> MKKESINTSGPDNTKSSISDEIEISNEISWTALSGVISAANNADGRLEVFGVGTNNAVWHNWQTVPNTGSSWSGWHSLNEGATSKPAVHINSDGRLEVFVRGTDNALWHNWQTVPGAGWSGWQSLGGQITSNPVVYINSDGRLEVFARGADNALWHIWQTAPHAGPWSNWQSLNGVLTSDPTVYVNASGRPEVFARSNDYSLWYIKQTASHTYPWTNWQSLSGVITSNPVVISNSDGRLEVFARGSDNALWHIWQVAPNAGWTNWRSLSGIITSDPAVHINADGRLEVFARGPDNALWHIWQTATSDAWSEWTSLSGVITSAPTVAKNSDGWLEVFARGANNALCHIQQTTSSWSTWTSLGGNLIDASAIK

In this article, we studied five members of the PLL lectin family from P. laumondii subsp. laumondii TT01 (PLL, PLL2, PLL3, PLL4, PLL5, collectively referred to as PLLs). All studied lectins belong to the seven-bladed β-propeller structural family. Each blade makes a W-motif composed of four antiparallel beta-strands (β1-β4) connected by β-turns and loops. The saccharide binding sites are located between the adjacent blades and are uniquely organized in two separate circles around the monomer.

The lowest avidity effect can be seen for PLL3, the only monomeric protein in this family. Residues involved in ligand binding are highly conserved throughout the PLL family. The orientation of the ligand in the H-type binding site is consistent across all PLLs (Fig. 8F - an example of PLL3-4H site). C6 of αMeFuc points inside the binding pocket, where it is stabilized via hydrophobic interaction. Two highly conserved tryptophans (e.g. W265 and W251 in PLL3-4H site) are essential in stabilizing the ligand via CH-π stacking interaction with C6, C5, and C4. Additional ligand stabilization is formed by a hydrogen bond between O3 and the side chain of the polar amino acid (Ser/Thr; e.g. S246 in PLL3-4H site) if presented in the β-turn T2. The methyl group on C1 of methyl-α-l-fucoside ligand is oriented towards the solvent, providing sufficient space to accommodate potential binding of methyl-β-l-fucoside in the H sites of PLLs. The ligand in the P-type binding site has a distinct orientation, where C6 is pointing outside the binding pocket (Fig. 8E - an example f PLL3-2P site). Delocalized electrons of the tryptophan (e.g. W111 in PLL3-2P site) are involved in the stabilization of C3, C4 and C5 via CH-π stacking interaction. In human blood activated by zymosan A, PLL2 and PLL3 inhibited ROS production, suggesting these lectins interfere with the innate immune system reaction in the early stages of the Photorhabdus infection. Different behaviour was seen for d-galactose, which inhibited only the binding of PLL3 and not PLL2, despite confirmed binding to both proteins from ITC, suggesting that d-galactose aims for different binding sites than MGMR in PLL2.> GATAEKQKHDGRVKIGHYILGDTLGVGTFGKVKVGKHELTGHKVAVKILNRQKIRSLDVVGKIRREIQNLKLFRHPHIIKLYQVISTPSDIFMVMEYVSGGELFDYICKNGRLDEKESRRLFQQILSGVDYCHRHMVVHRDLKPENVLLDAHMNAKIADFGLSNMMSDGEFLRTSCGSPNYAAPEVISGRLYAGPEVDIWSSGVILYALLCGTLPFDDDHVPTLFKKICDGIFYTPQYLNPSVISLLKHMLQVDPMKRATIKDIREHEWFKQDLPKYLFPEDPSYSSTMIDDEALKEVCEKFECSEEEVLSCLYNRNHQDPLAVAYHLIIDNRRIMNEAKDFYLATSPPDSFLDDHHLTRPHPERVPFLVAETPRARHTLDELNPQKSKHQGVRKAKWHLGIRSQSRPNDIMAEVCRAIKQLDYEWKVVNPYYLRVRRKNPVTST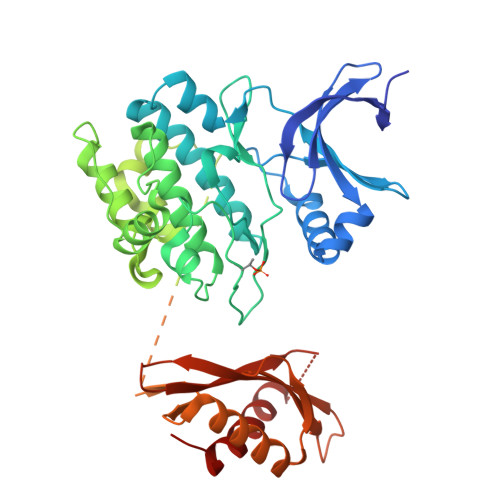FSKMSLQLYQVDSRTYLLDFRSIDDEASGGPGGSAPRPGSHTIEFFEMCANLIKILAQ>DYKDDDDKRPHSRLRQEDFPPRIVEHPSDVIVSKGEPTTLNCKAEGRPTPTIEWYKDGERVETDKDDPRSHRMLLPSGSLFFLRIVHGRRSKPDEGSYVCVARNYLGEAVSRNASLEVALLRDDFRQNPTDVVVAAGEPAILECQPPRGHPEPTIYWKKDKVRIDDKEERISIRGGKLMISNTRKSDAGMYTCVGTNMVGERDSDPAELTVFERPTFLRRPINQVVLEEEAVEFRCQVQGDPQPTVRWKKDDADLPRGRYDIKDDYTLRIKKTMSTDEGTYMCIAENRVGKMEASATLTVRAPPQFVVRPRDQIVAQGRTVTFPCETKGNPQPAVFWQKEGSQNLLFPNQPQQPNSRCSVSPTGDLTITNIQRSDAGYYICQALTVAGSILAKAQLEVTDVLTDRPPPIILQGPANQTLAVDGTALLKCKATGDPLPVISWLKEGFTFPGRDPRATIQEQGTLQIKNLRISDTGTYTCVATSSSGETSWSAVLDVTESGATISKNYDLSDLPGPPSKP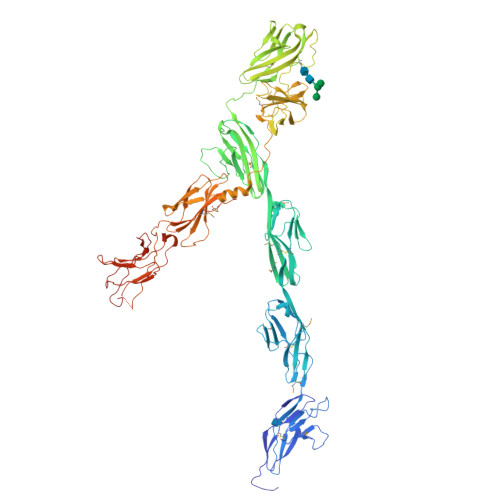QVTDVTKNSVTLSWQPGTPGTLPASAYIIEAFSQSVSNSWQTVANHVKTTLYTVRGLRPNTIYLFMVRAINPQGLSDPSPMSDPVRTQDISPPAQGVDHRQVQKELGDVLVRLHNPVVLTPTTVQVTWTVDRQPQFIQGYRVMYRQTSGLQATSSWQNLDAKVPTERSAVLVNLKKGVTYEIKVRPYFNEFQGMDSESKTVRTTEEAPSAPPQSVTVLTVGSYNSTSISVSWDPPPPDHQNGIIQEYKIWCLGNETRFHINKTVDAAIRSVIIGGLFPGIQYRVEVAASTSAGVGVKSEPQPIIIGRRNEVVITENNNSITEQITDVVKQPKLGSHHHHHH[3x]> MYGDLGNKLVLEAKRTKQLYARSNQDVNLPMYHEDIIRNILKEVSNLRKNTEYLKEQQQLGMLDDKVAKCQYF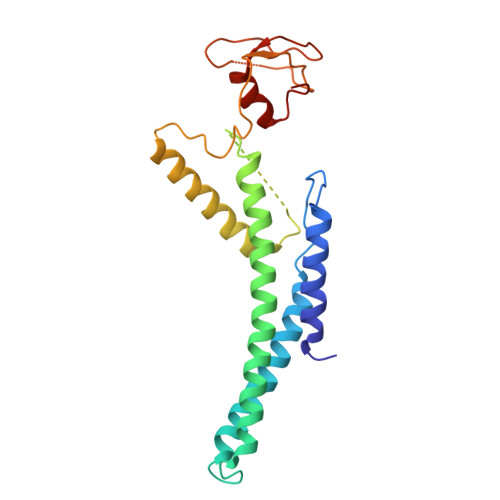VTLLCMERNKRCLLAYQRLRTDILDSMAWNNNGLDLMSSITFSQQDTNNLSHQEQEYLKEYCDLITDLKSGDLVDIDLSGSLVPPSDVFIDVRVLKDAGEIQTEYGVFNLIKDSQFFVRQSDVERLIQQGYLQKI> MRVSHEQFRAALQLVVSPGDPREYLANFIKIGEGSTGIVCIATEKHTGKQVAVKKMDLRKQQRRELLFNEVVIMRDYHHDNVVDMYSSYLVGDELWVVMEFLEGGALTDIVTHTRMNEEQIATVCLSVLRALSYLH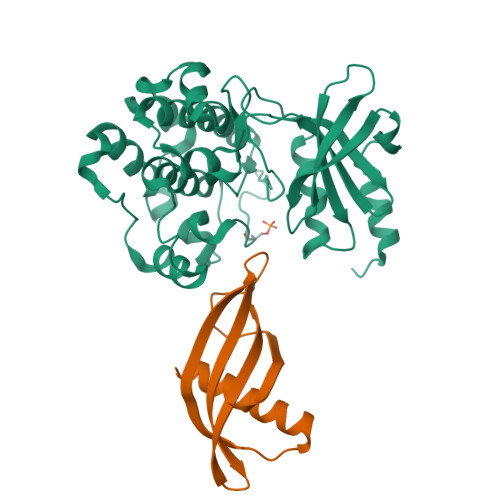NQGVIHRDIKSDSILLTSDGRIKLSDFGFCAQVSKEVPKRKSLVGTPYWMAPEVISRLPYGTEVDIWSLGIMVIEMIDGEPPYFNEPPLQAMRRIRDSLPPRVKDLHKVSSVLRGFLDLMLVREPSQRATAQELLGHPFLKLAGPPSCIVPLMRQYRHH;> MASNSLEIEELARFAVDEHNKKENALLEFVRVVKAKEQLVGWVYEFQTMYYLTLEAKDGGKKKLYEAKVWVKSDHMPPSLPNFKELQEFKPVGDAAAAHHHHHHHH> MSSDLVMPALGRPFTLGMLYDARREKLIPGFSLFGDETLQKYQSSNAQRSSEFKIVASDSTESKSSAMDIEASLGVSFLGGLVEVGGSAKYLNNTKKYQNQSRVTLKYKATTVYKQFTAPPGTVTVQETAITEKGLATHVVTSILYGANAFFVSDSDKVEDTNLQDIQGKMEAAIKKIPTISIEGSASVQLTDEEKSLASNLSCKFHGDFLLESLPTTFEDAVKTYQTLPTLIGEDGANSVPMKVWLAPLKSYNSKAQQLIQEINVSKVRRIHTTLEELHKLKRRANEAMDVKLVQRIPLIHDKISNFQQIFQDYMLTVQKKIAEKLPLVRAGTESEQSLQKIIDDRAQSPFSNEKVSKWLDAVEREIAVLKSCAGMVEGTQAKFVSNQTELDREVLVGKVKHAVCFIFTSVERNDPYLKVLSDYWESPPSNNAKDVAPSTEDKWCFSTEVVLKMQQRAQTFCDHVNDFEKSRNVGFFITALENGKFQGASIYYYKEGSLATQDFTFPRMPFVQGYKKRSDLLWYACDLTFDRNTINNWISLSDNDTFAASEHGKRQNYPKHPERFVSFNQVLCNEGLMGKHYWEVEWNGYIDVGIAYISIPRKEIDFASAFGYNTYSWVLSYNPKIGYIERHKKREYNVRAPNPGFKRLGLFLDWRYGSISFYAVSSDEVHHLHTFKTKFTEPVYPAFSIGPAGNHGTLRLL;> MPSDILVVAALGRPFTLGMLYDARNDKLIPGFTLWEDEVIEESTLESSQPSSAFEIIASDSTDDKSSLMDIEASLKASFLGGLVEVGGSAKYLNNQKKFKNQSRVTLQYKATTSFKQLMTNLGTKHVEYSELFENIQATHVVIGILYGANAFFVFDSNKVDSTNVQEIQGQMEAVIKKIPSVEISGKASVQLTGEETDITNSFSCEFHGDFFLTTNPTTFEDAVKTYQQLPQMMGKDNAVPMTVWLVPMVNFYSEAPQLMADSSTPILRKVRNTLEAIVQVQMRCNDALDDPTVNLFTEVQKKLSDFQKICDDHMSKLQATIAKKLFAIRSGDEDESALLNLFEENLQSPFNIESLNMWMEFEEREINVLRSCMDILTKAKPKVIFNQGVLFKGLYDSKVKHALCYVFTNVTKNDVFLNVLNEFLDSPQSRPKKLRPSPKDYWYSYDDIPETMREKAYLFRNLAKEMNNRCVHFFVTAIHNPKQEGAGIHYYRESIQIIDEFTKPYMPGVESIKDRRELQWYDCELTLDPETAHQ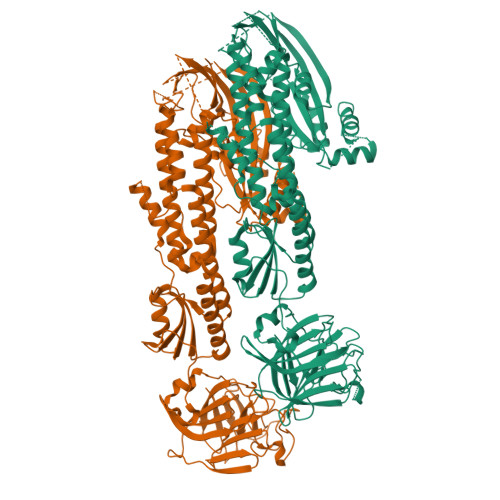VLTLSEGNKKAVSGNTKSPTDHLEKFSHFQQVMCTKGLSGRHYWELEWSGYVGAGVTYKGIGRKTSTSDSSLGKNEKSWLFEYSTKSGYQQIHNSKKTRVTVSSTGFKLLGVYLDWPAGTLSFYMVNKAWVTHLHTFHTKFNEAVYPAFLIGDAQQKVNGQIKLL> IDCDSSVFGNNFNITTSPQTLTMSGPLAPGKYQTTLTVQALIGGTGVVVGTVTFAGKTVAYQVFDDSFASFDLGTVTVSASTTPSVIWTGSTGATLTMAVNIICKPITPTSVAISGQPIWTTPY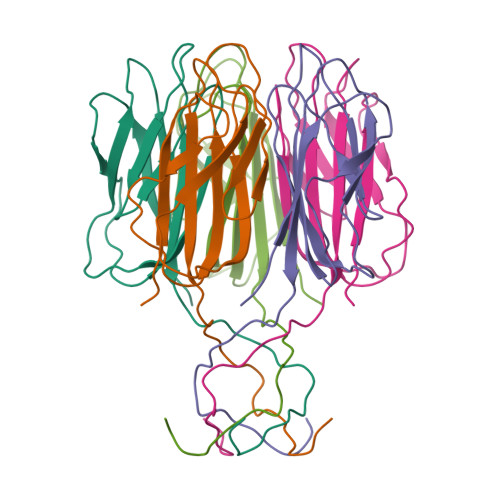AP>[2x]MSQRITIDPVTRIEGHLRIDCEIENGVVSKAWASGTMWRGMEEIVKNRDPRDAWMIVQRICGVC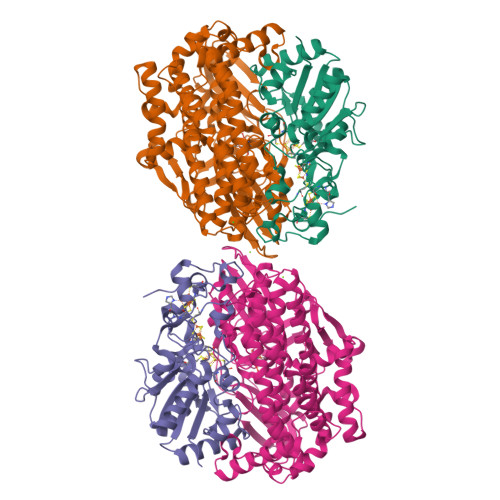TTTHALSSVRAAESALNIDVPVNAQYIRNIILAAHTTHDHIVHFYQLSALDWVDITSALQADPTKASEMLKGVSTWHLNSPEEFTKVQNKIKDLVASGQLGIFANGYWGHPAMKLPPEVNLIAVAHYLQALECQRDANRVVALLGGKTPHIQNLAVGGVANPINLDGLGVLNLERLMYIKSFIDKLSDFVEQVYKVDTAVIAAFYPEWLTRGKGAVNYLSVPEFPTDSKNGSFLFPGGYIENADLSSYRPITSHSDEYLIKGIQESAKHSWYKDEAPQAPWEGTTIPAYDGWSDDGKYSWVKSPTFYGKTVEVGPLANMLVKLAAGRESTQNKLNEIVAIYQKLTGNTLEVAQLHSTLGRIIGRTVHCCELQDILQNQYSALITNIGKGDHTTFVKPNIPATGEFKGVGFLEAPKGMLSHWMVIKDGIISNYQAVVPSTWNSGPRNFNDDVGPYEQSLVGTPVADPNKPLEVVRTIHSFDPCMACAVHVVDADGNEVVSVKVL;>MAESVTNPQRPPVIWIGAQECTGCTESLLRATHPTVENLVLETISLEYHEVLSAAFGHQVEENKHNALEKYKGQYVLVVDGSIPLKDNGIYCMVAGEPIVDHIRKAAEGAAAIIAIGSCSAWGGVAAAGVNPTGAVSLQEVLPGKTVINIPGCPPNPHNFLATVAHIITYGKPPKLDDKNRPTFAYGRLIHEHCERRPHFDAGRFAKEFGDEGHREGWCLYHLGCKGPETYGNCSTLQFCDVGGVWPVAIGHPCYGCNEEGIGFHKGIHQLANVENQTPRSQKPDVNAKEGGHHHHHH[2x]> RYNDYKLDFRRQQMQDFFLAHKDEEWFRSKYHPDEVGKRRQEARGALQNRLRVFLSLMETGWFDNLL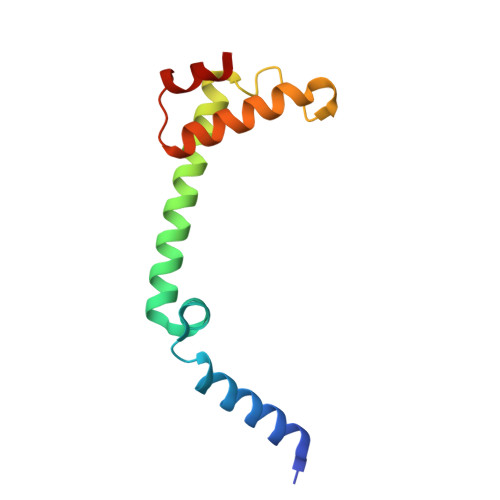LDIDKADAIVKMLDAAVIKMEGGTENDLRILEQ> MQPFGVLDRYIGKTIFTTIMMTLFMLVSLSGIIKFVDQLKKAGQGSYDALGAGMYTLLSVPKDVQIFFPMAALLGALLGLGMLAQRSELVVMQASGFTRMQVALSVMKTAIPLVLLTMAIGEWVAPQGEQMARNYRAQAMYGGSLLSTQQGLWAKD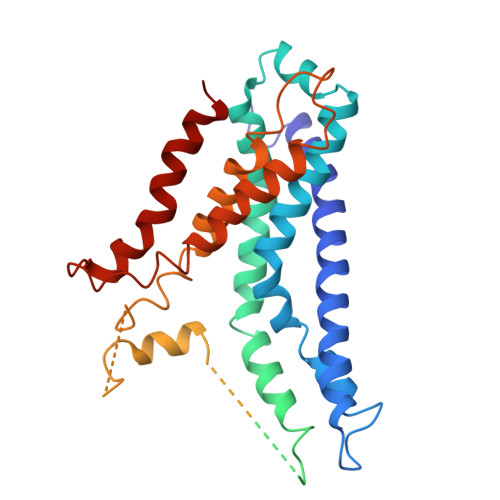GNNFVYIERVKGDEVLGGISIYAFNENRRLQSVRYAATAKFDPEHKVWRLSQVDESDLTNPKQITGSQTVSGTWKTDLTPDKLGVVALDPDALSISGLHNYVKYLKSSGQDAGRYQLNMWSKIFQPLSVAVMMLMALSFIFGPLRSVPMGVRVVTGISFGFVFYVLDQIFGPLTLVYGIPPIIGALLPSASFFLISLWLLMRKS>[2x]MGHHHHHHMYTDLKDKVVVITGGSTGLGRAMAVRFGQEEAKVVINYYNNEEEALDAKKEVEEAGGQAIIVQGDVTKEEDVVNLVQTAIKEFGTLDVMINNAGVENPVPSHELSLDNWNKVIDTNLTGAFLGSREAIKYFVENDIKGNVINMSSVHEMIPWPLFVHYAASKGGMKLMTETLALEYAPKGIRVNNIGPGAMNTPINAEKFADPVQRADVESMIPMGYIGKPEEVAAVAAFLASSQASYVT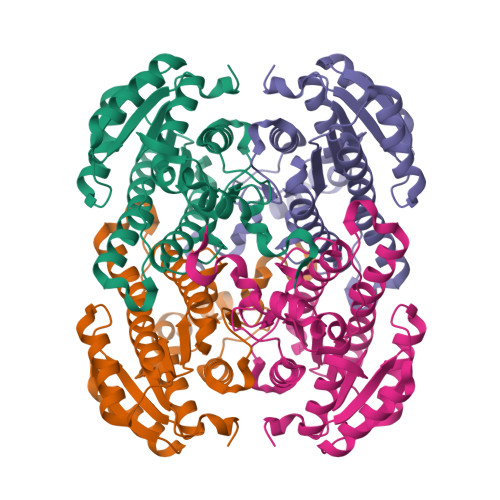GITLFADGGMTKYPSFQAGRG> TPQNITDLCA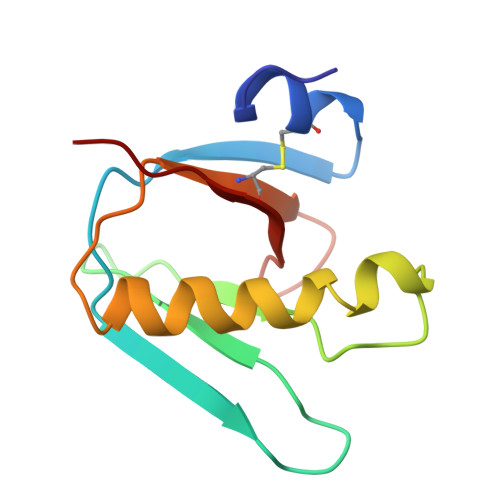EYHNTQIYTLNDKIFSYTESLAGKREMAIITFKNGAIFQVEVPSSQHIDSQKKAIERMKDTLRIAYLTEAKVEKLCTWNNKTPHAIAAISMAN> MNTVDPITLAVVRGALETAQREMTLTLEKTSRSSVFNLAHDYSNALFDHLPEMILQGQDIPIHLGSLIPAMKCVAGFFGDEIAEGDVIYHNDPAYMGSHILDCCMYKPVFYKGELVFWTVCKGHLTDIGGPVPAGYNPDAKEIYAEGLRIPPVKLWAQGQRREDVINLLLTNMRARAYQEGDLNAQYGACSVGERHLIELLDRYGVDQVRACITELKDMADRHMRALLRDVPDGFYSGTAILEDSGHGLGELSITAQVEIRGDEAHVLIESPPQVPYFINSYAGNSISGVYLGLMMFAQVPPPYNEGLYRCVSVDLGPSGTLCNAQEPAPHVNCTTTPMETLADAVRLALEQAAPERVTASWGHASGINIAGHDPRNNNDEYVTMVLASVISGAGANKAMDGWPACGPLCCFGALMSGDIELLEYSYPVLIHRYSLMTDSGGAGEFRGGSGTRLELEPLKHAMTVVGFGEGRQLPTAGAAGAKNVLLEPKLGRLIHRHVDGEEDHYIQNTLLTAQPGERVINVNPGGGGYGDPLRRPLATVLADVRNGLVSIDGARLEYGVVIDGNGQLDE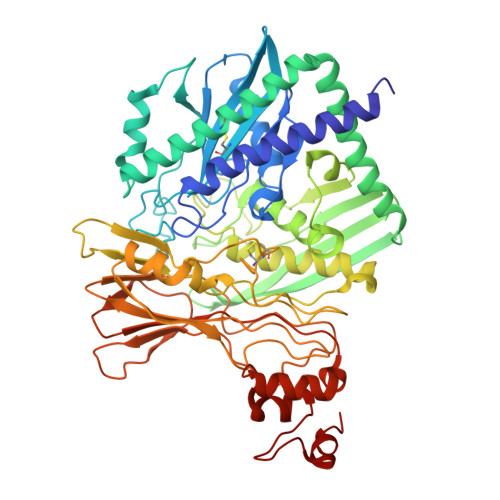AATHAHRAAH>[2x]ML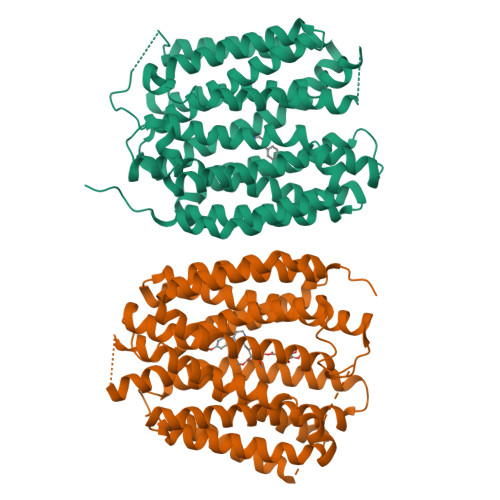RTILDAPQRLLKEGRASRQLVLVVVFVALLLDNMLFTVVVPIVPTFLYDMEFKEVNSSLHLGHAGSNCLQGTGFLEEEITRVGVLFASKAVMQLLVNPFVGPLTNRIGYHIPMFAGFVIMFLSTVMFAFSGTYTLLFVARTLQGIGSSFSSVAGLGMLASVYTDDHERGRAMGTALGGLALGLLVGAPFGSVMYEFVGKSAPFLILAFLALLDGALQLCILQPSKVSPESAKGTPLFMLLKDPYILVAAGSICFANMGVAILEPTLPIWMMQTMCSPKWQLGLAFLPASVSYLIGTNLFGVLANKMGRWLCSLIGMLVVGTSLLCVPLAHNIFGLIGPNAGLGLAIGMVDSSMMPIMGHLVDLRHTSVYGSVYAIADVAFCMGFAIGPSTGGAIVKAIGFPWLMVITGVINIVYAPLCYYLRSPPAKEEKLAILSQDCPMETRMYATQKPTKEFPLGEDSDEEPDHEE> D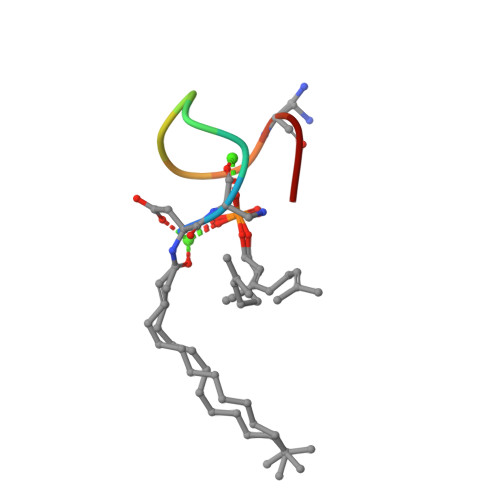AXDDGDGXIP> STLKKKRTWHKHGPGQAPDVKPVQNGSQLFIKELRSRTFPSAEDVVARVPGSQLTLGYMEEHGFTEPILVPKKDGLGLAVPAPTFYVSD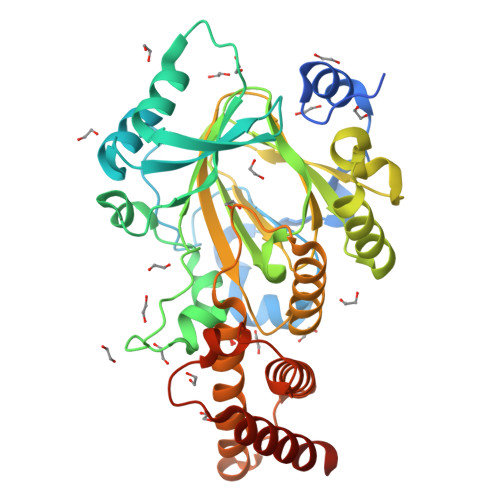VENYVGPERSVDVTDVTKQKDCKMKLKEFVDYYYSTNRKRVLNVTNLEFSDTRMSSFVEPPDIVKKLSWVENYWPDDALLAKPKVTKYCLICVKDSYTDFHIDSGGASAWYHVLKGEKTFYLIRPASANISLYERWRSASNHSEMFFADQVDKCYKCIVKQGQTLFIPSGWIYATLTPVDCLAFAGHFLHSLSVEMQMRAYEVERRLKLGSLTQFPNFETACWYMGKHLLEAFKGSHKSGKQLPPHLVQGAKILNGAFRSWTKKQALAEHEDELPEHFKPSQLIKDLAKEIRLSENASKAVRP> HHHHHHENLYFQGSGSSPRSGVLLRGCPTHCHCEPDGRMLLRVDCSDLGLSELPSNLSVFTSYLDLSMNNISQLLPNPLPSLRFLEELRLAGNALTYIPKGAFTGLYSLKVLMLQNNQLRHVPTEALQNLRSLQSLRLDANHISYVPPSCFSGLHSLRHLWLDDNALTEIPVQAFRSLSALQAMTLALNKIHHIPDYAFGNLSSLVVLHLHNNRIHSLGKKCFDGLHS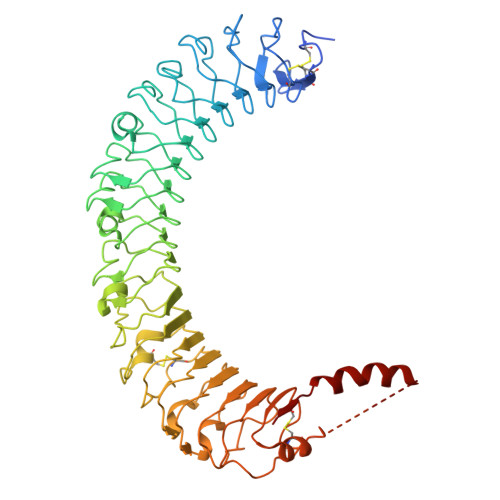LETLDLNYNNLDEFPTAIRTLSNLKELGFHSNNIRSIPEKAFVGNPSLITIHFYDNPIQFVGRSAFQHLPELRTLTLNGASQITEFPDLTGTANLESLTLTGAQISSLPQTVCNQLPNLQVLDLSYNLLEDLPSFSVCQKLQKIDLRHNEIYEIKVDTFQQLLSLRSLNLAWNKIAIIHPNAFSTLPSLIKLDLSSNLLSSFPITGLHGLTHLKLTGNHALQSLISSENFPELKVIEMPYAYQCCAFGVCENAYKISNQWNKGDNSSMDDLHKKDAGMFQAQDERDLEDFLLDFEEDLKALHSVQCSPAAA> ETGQCRIQKCTTDFVSLTSHLNSAVDGFDSEFCKALRAYAGCTQRTSKACRGNLVYHSAVLGISDLMSQRNCSKDGPTSSTNPEVTHG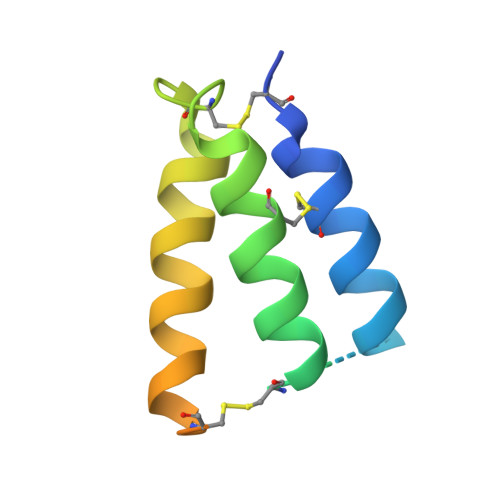TKHHHHHH> RKRTYETFKS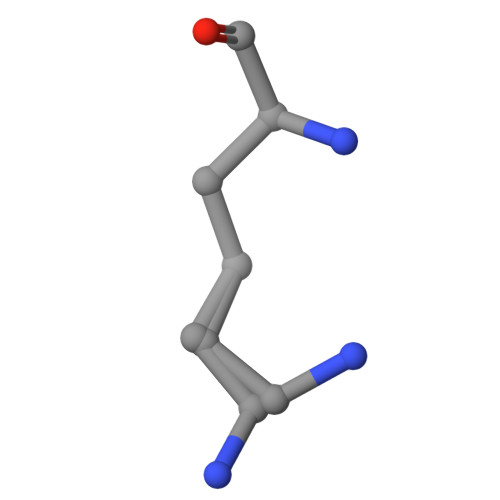IMKKS(4S)-N-[(1S,2R)-1-benzyl-3-{[3-(dimethylamino)benzyl]amino}-2-hydroxypropyl]-1-(3-methoxybenzyl)-2-oxoimidazolidine-4-carboxamide 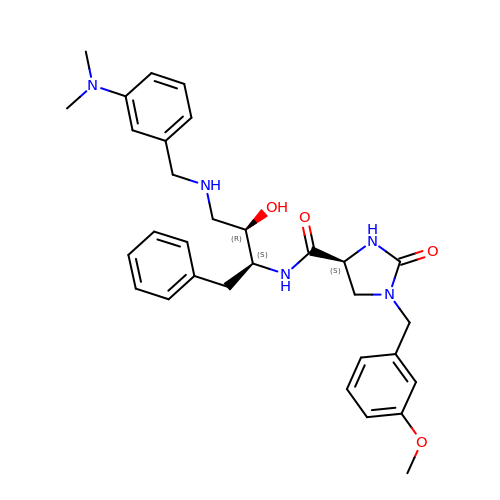| C31 H39 N5 O4 | MCBWJRZWLSXSBN-YTCPBCGMSA-N>SEWTGKSWMGKWESTDRIENFDAFISALGLPLEQYGGNHKTFHKIWKEGDHYHHQISVPDKNYKNDVNFKLNEEGTTQHNNTEIKYKYTEDGGNLKAEVHVPSRNKVIHDEYKVNGDELEKTYKVGDVTA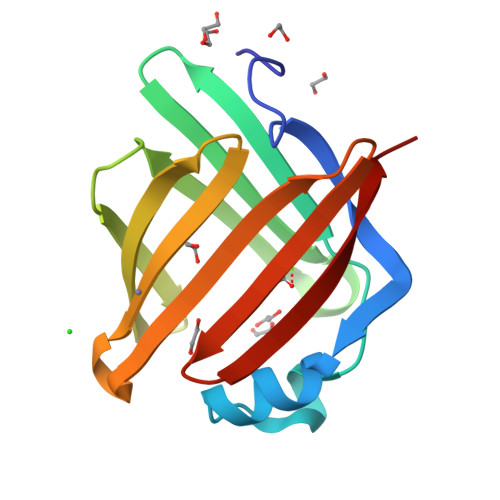KRWYKKSS[2x]GrlA and GrlR are two LEE-encoded regulators that are required to optimize PLEE1 activity. (2) GrlR, a negative regulator of ler expression, might act as anti-GrlA to establish an additional checkpoint that down-regulates the feedback loop, setting it back to the steady-state level. In agreement with this hypothesis, GrlR interacts with itself and also with GrlA to form a macromolecular assembly in the cytoplasm of AE pathogens. Here, we report the crystal structure of GrlR from EHEC refined up to 1.9 Å resolution as well as structure-based functional studies on GrlR.

The model was refined to a final R-factor of 0.215 (Rfree = 0.269) at 1.9 Å resolution with good stereochemical parameters. The GrlR model consists of residues from Met1 to Val111, with seven additional residues at the N-terminus (Gly-6, Leu-5, Val-4, Pro-3, Arg-2, Gly-1, and Ser0) resulting from the linker sequence of the (His)6 affinity tag. The C-terminal residues from Asn112 to Lys121 had no interpretable electron density and were not modeled. There are two molecules in the asymmetric unit and they are related by a 2-fold noncrystallographic symmetry approximately parallel to the a-axis. The GrlR molecule mainly consists of a single domain from residues Asp5 to Ile107 that forms a β-barrel. Residues Tyr59 to Asp70 form an extended loop that plugs one side of the cylindrical β-barrel structure. The β-barrel cavity is highly hydrophobic in nature with side chains from seven Tyr, six Ile, seven Leu, four Val, and two Phe residues lining the inner cavity surface. During structure refinement, we noticed a small molecule composed of 12 atoms in the hydrophobic cavity of GrlR, which, subsequently, was identified to be the fragment of Triton-X100. The strong hydrophobic cluster at the dimeric interface is maintained by the side chains from residues Ile7, Ile23, Ile25, Val39, and Ile107 from both monomers of the dimer. A loop region in the crystal structure of GrlR, residues Glu46 to Asp49 (46EDED49), is highly exposed on the surface and is less well defined in electron density.

>GLVPRGSMIMKDGIYSIIFISNEDSCGEGILIKNGNMITGGDIASVYQGVLSEDEDIILHVHRYNYEIPSVLNIEQDYQLVIPKKVLSNDNNLTLHCHVRGNEKLFVDVYAKFIEPLV[2x]>[5x]MASQDNIDHTASVIADTDNTIHQQAKAEERHRQAARRATQLRNDPVLSGINKLAFSV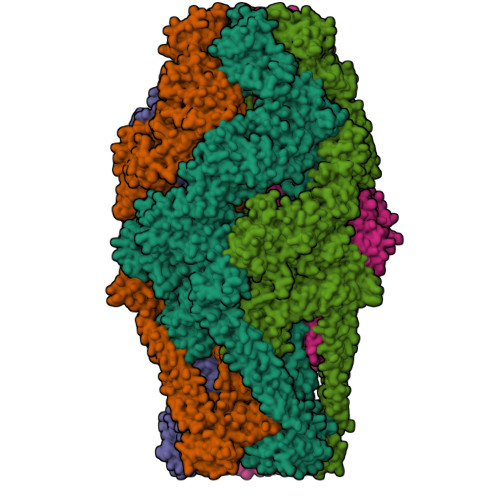APKILQPEARTDLSLAEGIPERANEYADPASIQSLFSPGRYLCELYHVAKELHEDGNKLHIDKRRPDLQDLVLNNSNMNQEVSSLEILLNVLQTKTPLDELTKDTEAHANDSSFTLPYDDNLTVINAILEDKAISLREIAVLLTEESDFSPTPALVQEQLGLNPASYALIDIKSPLDESYAKRLAHATQLSVEQLQWLNKNAIENSSNKNDPAKLEILAVISEYRRLHQRYGLSVDPFIAIINAVNTTHTNENKTSFFQQIFSTLDVDAGFNFLDQGSWEVIIRKALGITAEELLRIAKYCFGKSSISNVKMNSKKFSQLYRMAMIPRTLGVSFSQAEYLWQLYSHSDENIMEKIAQGNALTIIDAIIVLENTLQWMSEQKLDITTLQAMLTKQYSTTATPELFNFLSNIYQTLGKQVYSESLKPNLYRSLANGFHLKANVVAGLVNWLAKNDSEFTLERFWQNISMTFAEEPSLHQLEVHQPLLIQCQKLSQYVLIAQWAELSEQEIALILLPNGIDNRGSAPSPSITLLKLLSEFKLCQQEAKVSQSELFDIMQQLITDTNEKQEKLRNSADKVIRSIAKSIGSINNSMDDIDSTISIRNGSATLFPPEHPMYKALKLEVSNLEKSKIQLEGKKKEEEIKLEQAKDNIQSLINNWDSEIIIRLADAYHWDINIANSMFILIFGEKINFTFHYENRNDYHYEEHYGYRFEQKPMYSFDKKLTNGFGSILLLKNHIYIAEKLKIHPGTIIKIKNYIFDDKSNELENIANKLRVNLGSPTSTVLNKINESRRDALVNYYLAKNVSGDEKIKTAEQLYQYLLLDTKIGHEVKTSPIAEAISSLQIYINRCVDGEENDLHEKNISTHFSSDNFLHGWNSYNKRYARWAGKEKLMYYAADYIDPTLRYNKTELFNTFEQSINNSRLTEKSVKSALQSYLISYEKLAQIDTIKELYVENIKTHFFLGKTRESPCQYYWRSGEQLSNDSHHLRWSEWKKVECNINGTEEKFFINLSWYRNRLYVDWLNKTAFKTDEGKGKSEYHYNAAYKNDNNAWNDNISNMKIGLPWEQSKDIDEIPPIFINQDNVNSNSKNETYFITSGSTINNIPLFHGGYLEGEIKISFDKNKVKFTLEKPFERINEKSDYVIQINADMSDFNEIKNEKGESVTVEIKKNFNIMAYSLDEEYLGGNSFNRITFDTNIIHELDGDISLLPPDSLPLVEKLQTSVDELLSYSTQKDKIGLDAFSGSYGIYFWEFFFHIPFLASMRFLNEQRFDLAQHWLKYLLNSAGYRDRNGNLLKEGDNILYWNSLPLQQDTDWDKNTLTLPTDDPDVIAMQDPMQYKLAIFMRTLDLIISQGDQAYRQLERDTLAEAKIYYIQASQLLGSRPDLNRGHQWENIKLAEESRQAENGHFLPPYNEILLSYWDKLEIRLYNLRHNLNLDGQPLHLPLFATPVDPKALQRQHGAGNGINSGEQMATAQTSLYRFPLLIERAKSAVSSVIQFGNSLQSVLERQDNEAMTLLFQQQQQKVLQHTKDIQNNNIQVLQANLEATNSLKSAAKQRSKHYKELLDNGISSREQSGLDLRIDAGAVNIASVAPLMLAAALDTAPNVFGLADGGSHWGAVPYATSATLQISAGLTESRANINDIKANYDRREQEWTLQKNQADKDAEQLAHQYTSVQEQLNMAQKQRNLAELEQGHADALYQMQSTRFTGKELYNWMAGRLSGLYFQLFDATQPLCLMAKAVLEKEVDKAKTDGLFIRSGWNDLYQGLLAGEDLQLNLQKLENVWLMEEQRALEVERTVSLAQHYQQLSDHKFNLAEIVTGYMAQDKDQKTGNEQDFVELKNSTLIASLSIKGLNLVEDYPETMHLGDIRRIKQISVSLPALLGPYQDVQATLDYAGENTHLAKGCTALAISRGMNDSGQFQLDFNDGKYLPFEGIDISDKGTLVLRFPNATSKQKLLLQSLSDIILHIRYTIRS> MEQNRFKKETKTCSASWPRAPQSTLCATDRLELTYDVYTSAERQRRSRTATRLNLVFLHGSGMSKVVWEYY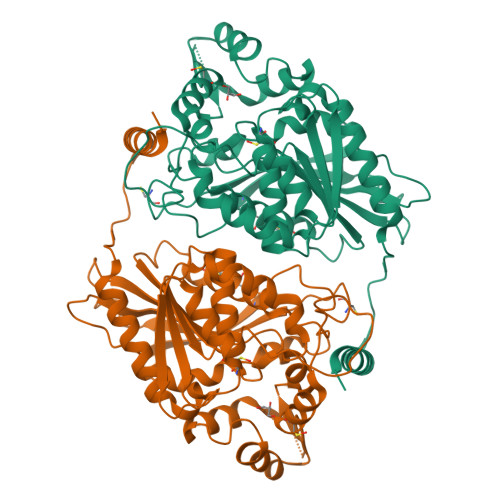LPRLVAADAEGNYAIDKVLLIDQVNHGDSAVRNRGRLGTNFNWIDGARDVLKIATCELGSIDSHPALNVVIGHSMGGFQALACDVLQPNLFHLLILIEPVVITRKAIGAGRPGLPPDSPQIPENLYNSLRLKTCDHFANESEYVKYMRNGSFFTNAHSQILQNIIDFERTKASGDDEDGGPVRTKMEQAQNLLCYMNMQTFAPFLISNVKFVRKRTIHIVGARSNWCPPQNQLFLQKTLQNYHLDVIPGGSHLVNVEAPDLVIERINHHIHEFVLTSPLQSSHIPQLTLEERAVMFDRAFDSFKNEALVKTTKQKLAAALEHHHHHH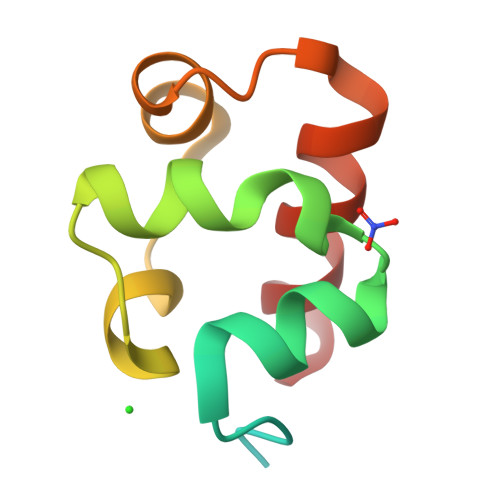>MHHHHHHSSGRENLYFQGDGIPYRTVSEWLESIRMKRYILHFHSAGLDTMECVLELTAEDLTQMGITLPGHQKRILCSIQGF[2x]> NINYFK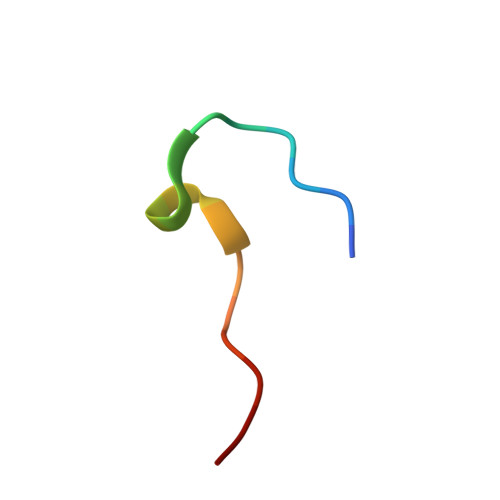DAASSGASRLD>RNGRAGPSDSAFSFTKSRARVLTEAPKVTFKDVAGAEEAKEELKEIVEFLKNPSRFHEMGARIPKGVLLVGPPGVGKTHLARAVAGEARVPFITASGSDFVEMFVGVGAARVRDLFETAKRHAPCIVFIDEIDAVGRKRGSGVGGGNDEREQTLNQLLVEMDGFEKDTAIVVMAATNRPDILDPALLRPGRFDRQIAIDAPDVKGREQILRIHARGKPLAEDVDLALLAKRTPGFVGADLENLLNEAALLAAREGRRKITMKDLEEAADRVMMLPAKKSLVLSPRDRRITAYHEAGHALAAHFLEHADGVHKVTIVPRGRALGFMMPRREDMLHWSRKRLLDQIAVALAGRAAEEIVFDDVTTGAENDFRQATELARRMITEWGMHPEFGPVAYAVREDTYLGGYDVRQYSEETAKRIDEAV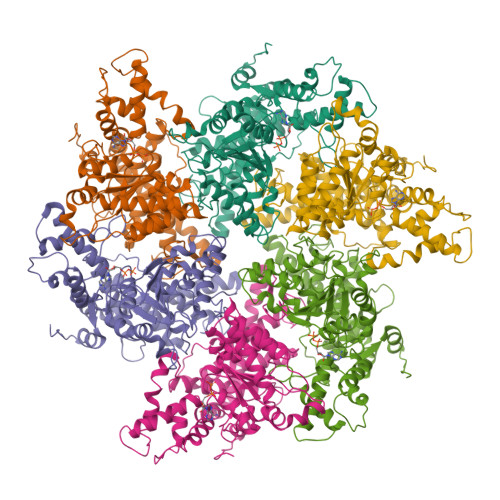RRLIEEQYQRVKALLLEKREVLERVAETLLERETLTAEEFQRVVEGLPLEAPEEAREEREPPRVVPKVKPGGALGGA[6x]>[2x]MAEEGTRSEAADAATQARQLPDSRNIFVSHRFPERQVDLGEVVMNFAEAGSPDNPALLLLPEQTGSWWSYEPVMGLLAENFHVFAVDIRGQGRSTWTPRRYSLDNFGNDLVRFIALVIKRPVVVAGNSSGGLLAAWLSAYAMPGQIRAALCEDAPFFASELVPAYGHSVLQAAGPAFEL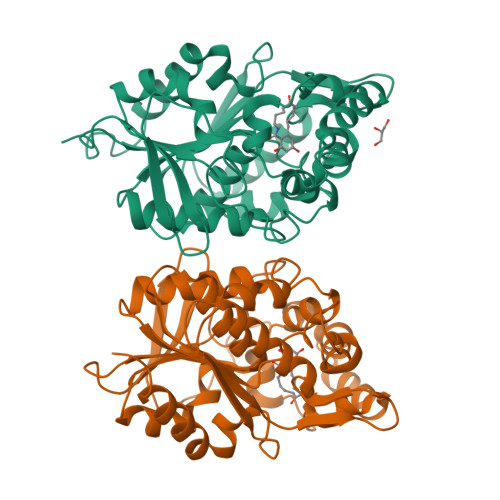YRDFLGDQWSIGDWKGFVEAAKASPAKAMQLFPTPDEAPQNLKEYDPEWGRAFFEGTVALHCPHDRMLSQVKTPILITHHARTIDPETGELLGALSDLQAEHAQDIIRSAGVRVDYQSHPDALHMMHLFDPARYAEILTSWSATLPANDHHHHHH N-(3-methylisothiazol-5-yl)-3-(1H-pyrazol-4-yl)imidazo[1,2-a]pyrazin-8-amine | C13 H11 N7 S | 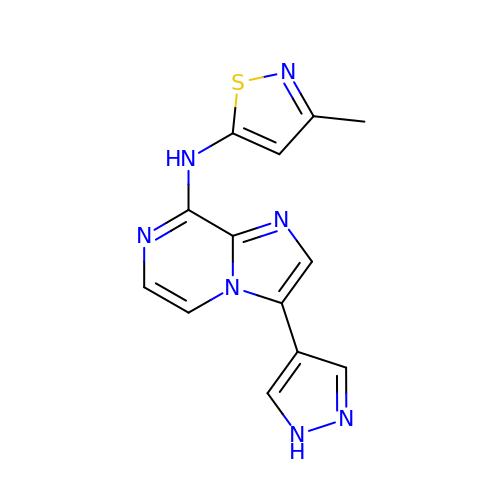XWFNCZUACYBPGT-UHFFFAOYSA-N>MGKRVVIALGGNALQQRGQKGSYEEMMDNVRKTARQIAEIIARGYEVVITHGNGPQVGSLLLHMDAGQATYGIPAQPMDVAGAMSQGWIGYMIQQALKNELRK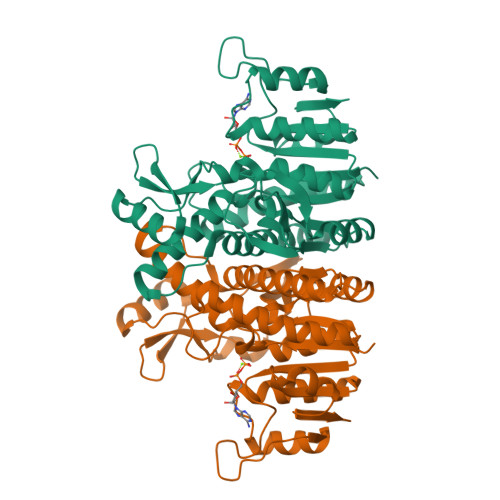RGMEKKVVTIITQTIVDKNDPAFQNPTKPVGPFYDEETAKRLAREKGWIVKEDSGRGWRRVVPSPDPKGHVEAETIKKLVERGVIVIASGGGGVPVILEDGEIKGVEAVIDKDLAGEKLAEEVNADIFMILTDVNGAALYYGTEKEQWLREVKVEELRKYYEEGHFKAGSMGPKVLAAIRFIEWGGERAIIAHLEKAVEALEGKTGTQVLP[2x]> CPRFLKVKNWETDVVLTDTLHLKSTLETGCTEHICMGSIMLPSQHTRKPEDVATKDQLFPLAKEFLDQYYSSIKRFGSKAHMDRLEEVNKEIESTSTYQLKDTELIYGAKHAWRNASRCVGRIQWSKLQVFDARDCTTAHGMFNYICNHVKYATNKGNLRSAITIFPQRTDGKHD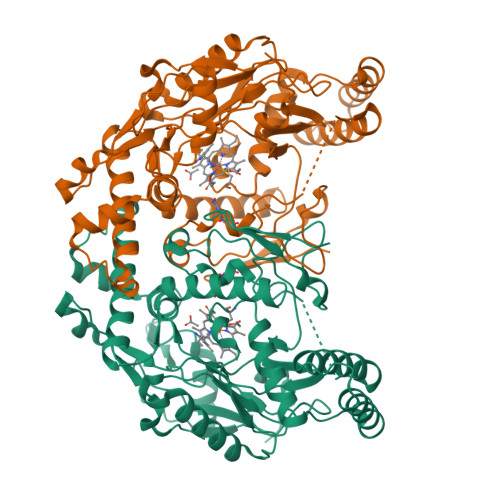FRVWNSQLIRYAGYKQPDGSTLGDPANVQFTEICIQQGWKAPRGRFDVLPLLLQANGNDPELFQIPPELVLEVPIRHPKFDWFKDLGLKWYGLPAVSNMLLEIGGLEFSACPFSGWYMGTEIGVRDYCDNSRYNILEEVAKKMDLDMRKTSSLWKDQALVEINIAVLYSFQSDKVTIVDHHSATESFIKHMENEYRCRGGCPADWVWIVPPMSGSITPVFHQEMLNYRLTPSFEYQPDPWNTHVWKL>SVDREEMIERFANFLREYTDEDGNPVYRGKITDLL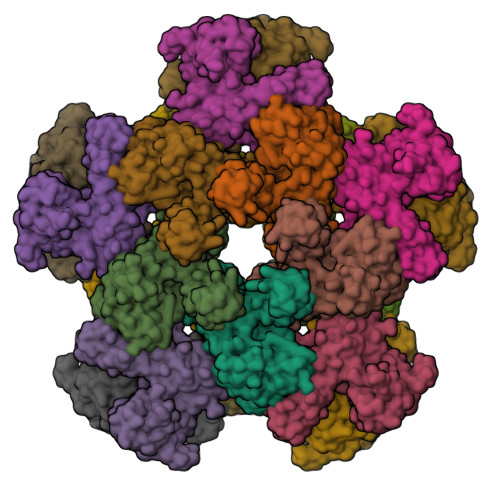TITPKRSVAIDWMHLNSFDSELAHEVIENPEEGISAAEDAIQIVLREDFQREDVGKIHARFYNLPETLMVKDIGAEHINKLIQVEGIVTRVGEIKPFVSVAVFVCKDCGHEMIVPQKPYESLEKVKKCEQCGSKNIELDVNKSSFVNFQSFRIQDRPETLKGGEMPRFIDGILLDDIVDVALPGDRVIVTGILRVVLEAAEATPIFRKILEVNHIEPVSKEI[10x]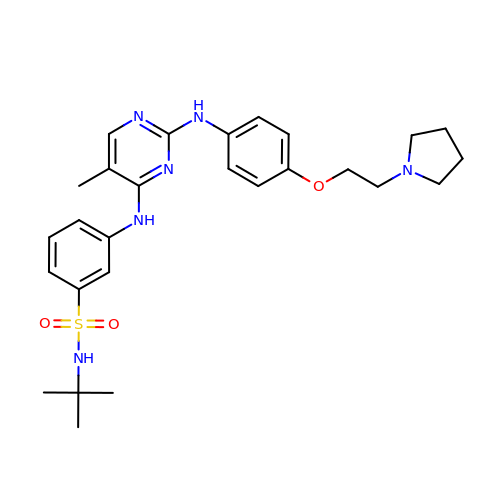N-tert-butyl-3-{[5-methyl-2-({4-[2-(pyrrolidin-1-yl)ethoxy]phenyl}amino)pyrimidin-4-yl]amino}benzenesulfonamide | C27 H36 N6 O3 S | JOOXLOJCABQBSG-UHFFFAOYSA-N>[12x]MAKKTSSTVLPFEAMPQHPGNRWLRLLQIWREQGYEHLHLEMHQTFQELGPIFRYNLGGPRMVCVMLPEDVEKLQQVDSLHPCRMILEPWVA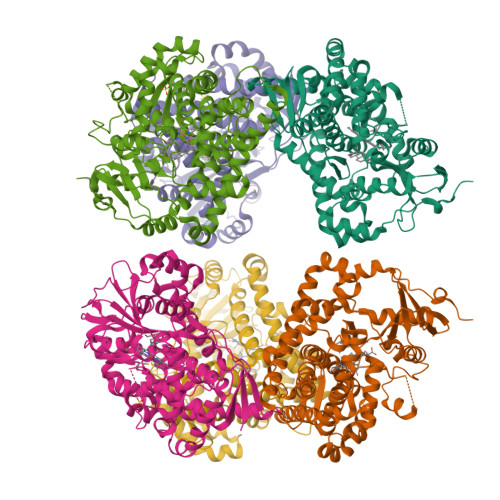YRQHRGHKCGVFLLNGPEWRFNRLRLNPDVLSPKAVQRFLPMVDAVARDFSQALKKKVLQNARGSLTLDVQPSIFHYTIEASNLALFGERLGLVGHSPSSASLNFLHALEVMFKSTVQLMFMPRSLSRWISPKVWKEHFEAWDCIFQYGDNCIQKIYQELAFNRPQHYTGIVAELLLKAELSLEAIKANSMELTAGSVDTTAFPLLMTLFELARNPDVQQILRQESLAAAASISEHPQKATTELPLLRAALKETLRLYPVGLFLERVVSSDLVLQNYHIPAGTLVQVFLYSLGRNAALFPRPERYNPQRWLDIRGSGRNFHHVPFGFGMRQCLGRRLAEAEMLLLLHHVLKHFLVETLTQEDIKMVYSFILRPGTSPLLTFRAINHHHHHH3-[[(2~{R},3~{S},4~{R},5~{R})-5-[8-[3-[[(2~{R},3~{S},4~{R},5~{R})-5-(6-aminopurin-9-yl)-3,4-bis(oxidanyl)oxolan-2-yl]methyl-(2-azanylethyl)amino]prop-1-ynyl]-6-azanyl-purin-9-yl]-3,4-bis(oxidanyl)oxolan-2-yl]methylamino]-3-oxidanylidene-propanoic 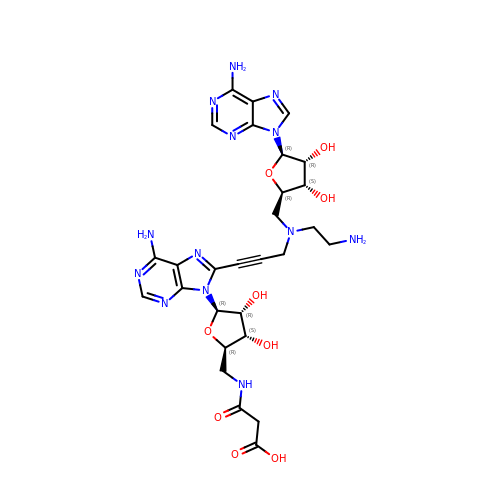acid | C28 H35 N13 O9 | SROHEFTVUSADJE-QJYUSYPVSA-N>MEKTRTEPSIWTVDDVWAFIHSLPGCQDIADEFRAQEIDGQALLLLKEDHLMSAMNIKRGPALKICA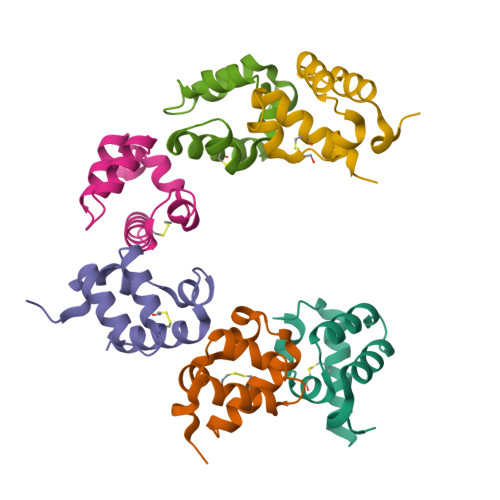RINSLKESRHHHHHH[6x]In Gram-positive bacteria, nitrogen homeostasis is controlled by an operon encoding glutamine synthetase (GS), a dodecameric machine that assimilates ammonium into glutamine, and the GlnR repressor. GlnR detects nitrogen excess indirectly by binding glutamine-feedback-inhibited-GS (FBI-GS), which activates its transcription-repression function. GS generates glutamine from glutamate, ATP, and ammonium by a mechanism that involves the initial phosphorylation of the γ-carboxyl group of glutamate by ATP and the subsequent incorporation of ammonium. The structures show FBI-GS binds the GlnR C-terminal domain within its active-site cavity, juxtaposing two GlnR monomers to form a DNA-binding-competent GlnR dimer.

We next obtained structures of Sa GlnR and Lm GlnR bound to a 21 bp glnR consensus operator site to 2.35 and 3.45 Å, respectively, by X-ray crystallography. The Lm and Sa GlnRs form comparable dimers to the Bs GlnR and dock on the DNA similarly. As observed in the Bs structure, both DNA sites bound by Sa and Lm GlnR are bent inward but the DNA from the Lm complex is slightly less bent (~21°) compared to the Sa and Bs structures (~25°). However, like Bs GlnR, the Sa and Lm GlnR surfaces that contact the DNA are both electropositive, indicating electrostatics as a general contributor to GlnR DNA binding. The GlnR DNA used for crystallization contains four conserved bps (bolded) in each half-site, 5′-CGTGTCAGATAATCTGACACG-3′ (where the consensus binding site is N1N2T3G4T5N6A7N(7)T7’N6’A5’C4’A3’N2’N1’; N indicates any nucleotide). These conserved bps are contacted in the major groove by Lm and Sa GlnR residues that are completely conserved among GlnRs; a conserved tyrosine (Sa Tyr32/Lm Tyr31) makes hydrophobic contacts to the DNA thymine3 (T3) methyl group, an arginine (Sa Arg28/Lm Arg27) specifically reads the G4 base and makes hydrophobic interactions with the methyl moiety of T5 and finally, the side chain methylene carbons of a conserved arginine (Sa Arg31/Lm Arg30) contacts the T7′ methyl group. However, GlnR proteins contain different wing residues, which our structures show make distinct contacts to the minor groove; wing residues Bs Arg46 and Sa Lys48 make nonspecific base contacts in the minor groove, but the corresponding Lm GlnR residue, His47, makes hydrophobic contacts to a ribose. To test the role of this wing residue in operator DNA-binding affinity, we mutated the Sa GlnR Lys48 residue to arginine and histidine, which are found in Bs and Lm GlnR and performed FP studies. The Kds determined in these experiments were 9.9 ± 0.8 nM, 8.0 ± 0.6 nM, and 11.6 ± 0.6 nM for WT Sa GlnR(1-87), Sa GlnR(1-87)K48R, and Sa GlnR(1-87)K48H, respectively. Thus, these data indicate that the different wing contacts by GlnR proteins do not significantly impact operator binding affinity. The Sa GlnR dimer is generated by interacting N-terminal loops, while the Lm and the Bs N-terminal regions fold into distorted helices that interact.

>GSHMISNDAIRRNMAVFSMSVVSKLTDLTPRQIRYYETHELIKPERTEGQKRLFSLNDLERLLEIKSLLEKGFNIKEIKQIIYDSQ[4x]> GAMSETSVNRGPEKIRPECFELLRVLGKGGYGKVFQVRKVTGANTGKIFAMKVLKKAMIVRNAKDTAHTKAERNILEEVKHPFIVDLIYAFQTGGKLYLILEYLSGGELFMQLEREGIFMEDTACFYLA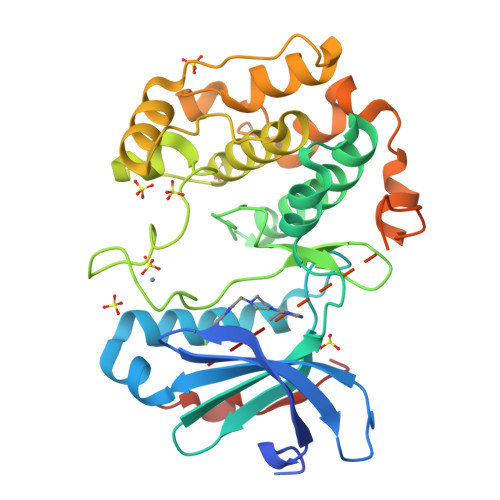EISMALGHLHQKGIIYRDLKPENIMLNHQGHVKLTDFGLCKESIHDGTVTHTFCGTIEYMAPEILMRSGHNRAVDWWSLGALMYDMLTGAPPFTGENRKKTIDKILKCKLNLPPYLTQEARDLLKKLLKRNAASRLGAGPGDAGEVQAHPFFRHINWEELLARKVEPPFKPLLQSEEDVSQFDSKFTRQTPVDSPDDSTLSEEEQEMFRDFEYIADW>SMTDQAFVTLTTNDAYAKGALVLGSSLKQHRTTRRLVVLATPQVS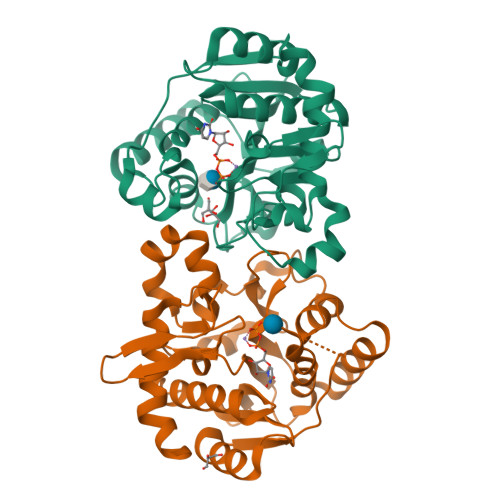DSMRKVLETVFDEVIMVDVLDSGDSAHLTLMKRPELGVTLTKLHCWSLTQYSKCVFMDADTLVLANIDDLFDREELSAAPDPGWPDCFNSGVFVYQPSVETYNQLLHLASEQGSFDGGDQGILNTFFSSWATTDIRKHLPFIYNLSSISIFSYLPAFKVFGASAKVVHFLGRVKPWNYTYDPKTKSVKSEAHDPNMTHPEFLILWWNIFTTNVLPLLQ[2x]> MFDYETLRFIWWLLIGVILVVFMISDGFDMGIGCLLPLVARNDDERRIVINSVGAHWEGNQVWLILAGGALFAAWPRVYAAAFSGFYVAMILVLCSLFFRPLAFDYRGKIADARWRKMWDAGLVIGSLVPPVVFGIAFGNLLLGVPFAFTPQLRVEYLGSFWQLLTPFPLLCGLLSLGMVILQGGVWLQLKTVGVIHLRSQLATKRAALLVMLC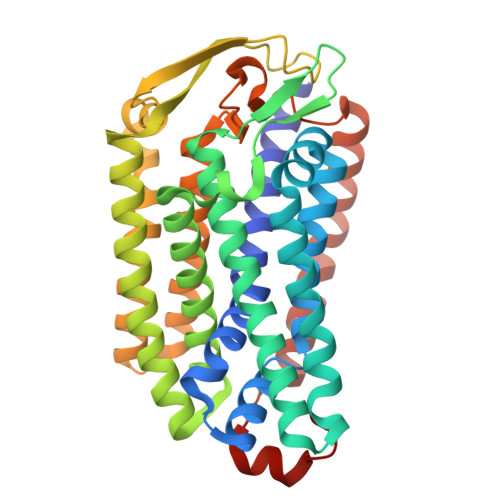FLLAGYWLWVGIDGFVLLAQDANGPSNPLMKLVAVLPGAWMNNFVESPVLWIFPLLGFFCPLLTVMAIYRGRPGWGFLMASLMQFGVIFTAGITLFPFVMPSSVSPISSLTLWDSTSSQLTLSIMLVIVLIFLPIVLLYTLWSYYKMWGRMTTETLRRNENELY We have used a glycoside hydrolase from Bacteroides thetaiotaomicron, BtGH84,17 as a model system to explore activation by small molecules. The catalytic domain of BtGH84 is homologous to that of the human enzyme O-GlcNAcase (OGA) which removes the N-acetylglucosamine post-translational modification on serine and threonine amino acids and BtGH84 itself indeed functions as a generic hexosaminidase. Using a bacterial glycoside hydrolase, BtGH84, we demonstrate how small molecule “fragments”, identified as activators in free solution, can be covalently tethered to the protein using Michael-addition chemistry. We show how tethering generates a constitutively-activated enzyme-fragment conjugate, which displays both improved catalytic efficiency and increased susceptibility to certain inhibitor classes.

We noted that position 2 on the quinazoline ring of 3 presented a vector towards Cγ of Y550, positioned on a flexible loop above the enzyme active site. We designed tethering compound 4, which we predicted would undergo Michael-style conjugate addition to the acrylamide from the free cysteine thiol introduced by the mutation Y550C. In order to direct reactivity of 4 with BtGH84 to the desired site, a triple mutant (Y550C, C420S, C654S, hereafter BtGH84_TM – signifying triple mutant) was expressed. In the absence of an inhibitor in this structure the active site is occupied by ethylene glycol. Compounds 9 and 10 attempt to coordinate the water seen H-bonded to H433 in the structure of BtGH84_TM-4, potentially stabilising the conformation seen in this structure and reducing linker mobility. The quinazoline ring is seen stacking onto Y137 and pointing towards the active site, with the amide linker coordinating a water molecule with Q551. The varying position of the tether in these three structures demonstrates the flexibility of the linker, however the fragment is in each case centred on the π-stacking interaction with Y137 (ESI Fig. 9†).

> MGSSHHHHHHQWNVSLQPPPQQLIVQNKTIDLPAVYQLNGGEEANPHAVKVLKELLSGKQSSKKGMLISIGEKGDKSVRKYSRQIPDHKEGYYLSVNEKEIVLAGNDERGTYYALQTFAQLLKDGKLPEVEIKDYPSVRYRGVVEGFYGTPWSHQARLSQLKFYGKNKMNTYIYGPKDDPYHSAPNWRLPYPDKEAAQLQELVAVANENEVDFVWAIHPGQDIKWNKEDRDLLLAKFEKMYQLGVRSFAVFFDDISGEGTNPQKQAELLNYIDEKFAQVKPDINQLVMCPTEYNKSWSNPNGNYLTTLGDKLNPSIQIMWTGDRVISDITRDGISWINERIKRPAYIWWNFPVSDYVRDHLLLGPVYGNDTTIAKEMSGFVTNPMEHAESSKIAIYSVASYAWNPAKYDTWQTWKDAIRTILPSAAEELESFAMHNSDLGPNGHGYRREESMDIQPAAERFLKAFKEGKNYDKADFETLQYTFERMKESADILLMNTENKPLIVEITPWVHQFKLTAEMGEEVLKMVEGRNESYFLRKYNHVKALQQQMFYIDQTSNQNPCQPGVKTATRVIKPLIDRTFATVVKFFNQKFNAHLDATTDYMPHKMISNVEQIKNLPLQVKANRVLISPANEVVKWAAGNSVEIELDAIYPGENIQINFGKDAPSTWGRLEISTDGKEWKTVDLKQKESRLSAGLQKAPVKFVRFTNVSDEEQQVYLRQFVLTIEKK> MYEMFLFNSVNSKITQNVNEEFILKYSDYSCEQLNSLWKEVGLGSYYNGLFKIIEPNDLKDIINQCYIMDDDESLLPFMCTAFG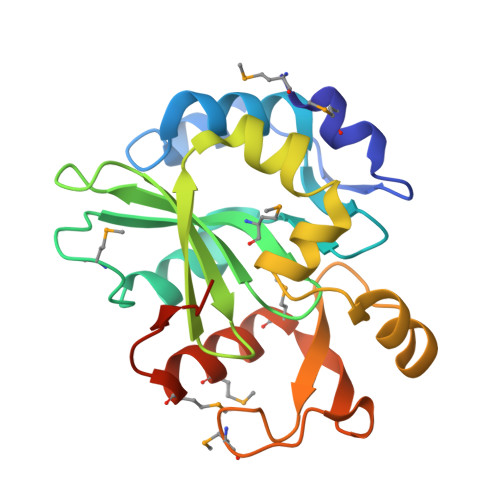DVFAYVKNKRFGNYVVFLNIRYGTSLIIPDNFVAIFNKVIPNQSFLKGWFDLENYAFVKEKIGEIDFDECYGYFPTLSMGGNESIDNISIVKMIPYIDMNVQMIDVFERADKHHHHHH>SQNGRIDPFTLVLGPLYAIDAPFAVNLVSQNGRRYLKASISLELSNEKLLNEVKVKDTAIKDTIIEILSSKSVEEVVTNKGKNKLKDEIKSHLNSFLIDGFIKNVFFTDFIIQ[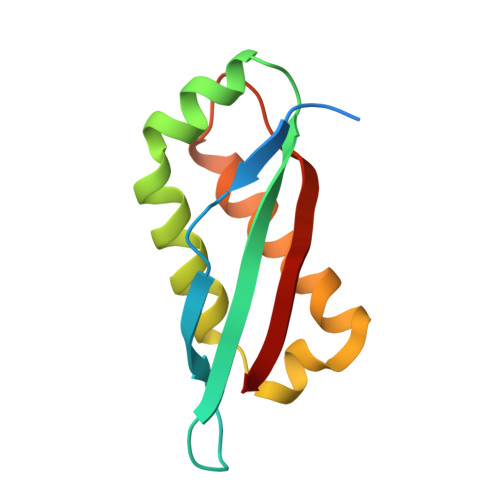12x]>PKKQTRLGLEAKKEENLADWYSQVITKSEMIEYHDISGCYILRPWAYAIWEAIKDFFDAEIKKLGVENCYFPMFVSQSALEKEKTHVADFAPEVAWVTRSGKTELAEPIAIRPTSETVMYPAYAKWVQSHRDLPIKLNQWCNVVRWEFKHPQPFLRTREFLWQEGHSAFATMEEAAEEVLQILDLYAQVYEELLAIPVVKGRKTEKEKFAGGDYTTTIEAFISASGRAIQGGTSHHLGQNFSKMFEIVFEDPKIPGEKQFAYQNSWGLTTRTIGVMTMVHGDNMGLVLPPRVACVQVVIIPCGITNALSEEDKEALIAKCNDYR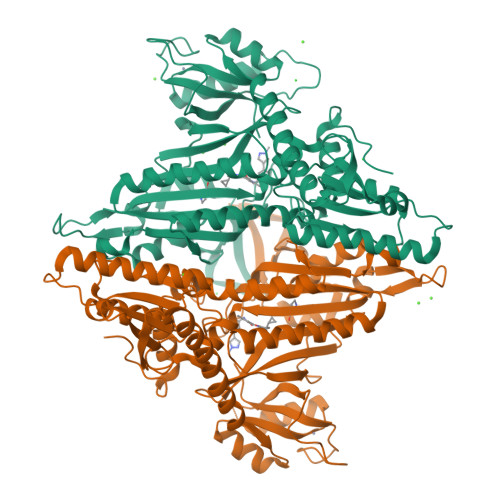RRLLSVNIRVRADLRDNYSPGWKFNHWELKGVPIRLEVGPRDMKSCQFVAVRRDTGEKLTVAENEAETKLQAILEDIQVTLFTRASEDLKTHMVVANTMEDFQKILDSGKIVQIPFCGEIDCEDWIKKTTARDQDLEPGAPSMGAKSLCIPFKPLCELQPGAKCVCGKNPAKYYTLFGRSY[2x]> SMGVTSAETLTIATVNNGDMIRMQKLTDDFTKKNPGIDVKWVTLEENVLRQKVTTDVATKGGQYDVMTIGIYEAPIWGKQGWLAPL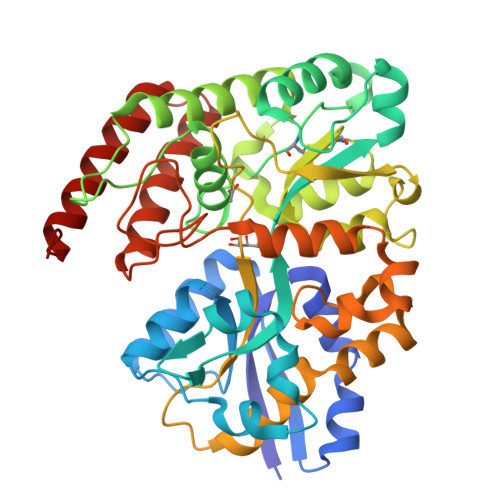DKLSADKDYDAADLLPPVRSGLTVDGKLYAAPFYAESSMVMYRKDLFEKAGLKMPEAPTWDFIKEAADKITDKSKEVYGICLRGKAGWGENIAFLSAMSNSFGARWFDEQWKPQFDQPEWKKTLQFYVDLMKKNGPPGASSNGFNENLALFQTGKCGMWIDATVAASFVTNPKESKVADQVGFALAPDNGLGKRGNWLWSWNLAIPAGSKKVEAAEKFIAWATSKDYLKLVAEKDGWANVPPGTRTSLYANADYQKAAPFAKMTLDSINSADPKHPTVKPVPYEGVQYVAIPEFQGIGTAVGQQFSAALAGQTTVDQALKTAQTLTEREMKKAGYPKK>MRGSHHHHHHGSMQILLANPRGFCAGVDRAISIVENALAIYGAPIYVRHEVVHNRYVVDSLRERGAIFIEQISEVPDGAILIFSAHGVSQAVRNEAKSRDLTVFDATCPLVTKVHMEVARASRRGEESILIGHAGHPQVEGTMGQYSNPEGGMYLVESPDDVWKLTVKNEEKLSFMTQTTLSVDDTSDVIDALRKRFPKIVGPRKDDICYATTNRQEAVRALAEQAEVVLVVGSKNSSNSNRLAELAQRMGKRAFLIDDAKDIQEEWVKEVKCVGVTAGASAPDILVQNVVARLQQLGGGEAIPLEGREENIVFEVPKE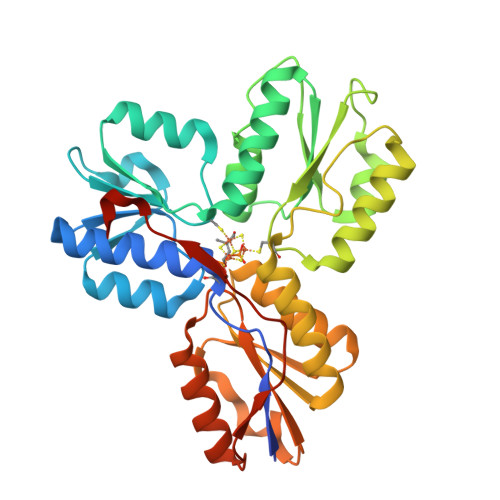LRVDIREVD[2x]The G•U wobble base pair is the most frequent among the non-WC base pairs in RNA molecules. The G•U pairs can be accommodated within A-form RNA helices with minimal structural distortions. The types of G•U tandems vary in terms of their structural, electrostatic, and thermodynamic properties. The negatively polarized surface within the major groove of the G•U wobble pair has a strong affinity for divalent metal ions.

In this work, we present the crystal structure of an RNA 8-mer duplex r[UCGUGCGA]2, providing detailed structural insights into the tandem motif I (5′UG/3′GU) complexed with Ba2+ cation. The crystals in the H32 space group, with one duplex in the asymmetric unit, diffracted X-rays to 2.2 Å resolution. Structural analysis of the presented RNA duplex confirmed the A-form helix and indicated a few unique features of the G•U tandem. The obtained electron density maps allowed tracing RNA unambiguously and modeling one Ba2+ cation and two water molecules in its coordination sphere. The strong peak (9.9σ level) in the anomalous difference electron density map corroborated the presence of Ba2+; at the used X-ray energy of 12,400 eV, the f′′ of barium is ∼4.1e. Ba2+ was bound in the duplex major groove by the exo-O4 atoms of U4 residues in both chains and the O6 atom of G5 (chain A). Two water molecules coordinated Ba2+ in the major groove. The major groove of the presented helix, also containing motif I wobble tandem, revealed a direct inter-strand phosphate–phosphate distance of 16.5 Å. Moreover, analysis of the surface electrostatic potential of this duplex indicated the presence of a negatively charged region within the major groove, which was, in fact, the Ba2+ cation binding site. Since the G•U tandem represents motif I, the 5′UG/3′GU tandem base-pair step had a high twist angle of 40.3°, while the steps between the wobble tandem and the flanking WC base pairs (5′GU/3′CG and 5′GC/3′UG) exhibited lower than average twist angles of 27.1° and 27.6°.

>[2x]UCGUGCGA> MTEKKRSTTQRAKKAAKTADVATLDATPQNPSALGGGLEGAERNTREMFRWTPAIISPDQQIAQDGTLALSRAQDIVQNDGYAFGAVAIHRDSVVGSQYKLNSKPNSLVLGAPEGWAEEFQEVVEARFNMVAESPENWFDARRMNTLTGLVRLAVGGFIMTGEVLASCEWMKPNGTRMQRRPFGTAIQMISPYRLSNPDNIMDDKYLRSGVKLDEMGAPIGYWLRKAFPGDPTDLEQWRWEYQPARFDWGRRRMIHIIEALLPGQTRGISEMVAALKQMKMTRNFQEVTLQNAIVNATYAAAIESELPSDVVFNQMGMGQTPFGDILKTYMGSLAEYIAGSKNIAIDGAKIPHLFPGTKLKMQPAGTPGGVGTDYEESLLRNIAASLGLSYEQFSRDYTKTNYSSARASMAETWKYMESRKKLVADRFASMIYTLWLEEEVNAGNVPLPPGFTWRDFYDPMKRDALCNAEWIGASRGQIDEKKETEAAILRIKNGLSTYEAEIARLGGDFREVFKQRAREEGIIKDLGLDFSGKMV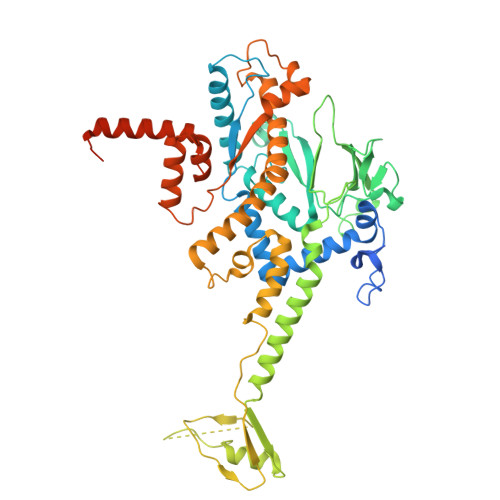EGTEASGSTGSTGSDNNNEEDTKE9-METHYL-9H-PURIN-6-AMINE 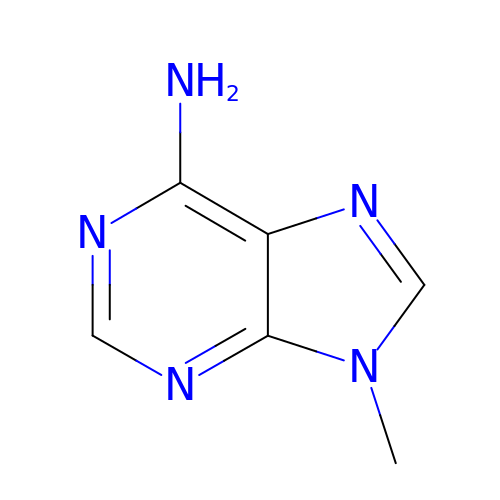| C6 H7 N5 | WRXCXOUDSPTXNX-UHFFFAOYSA-N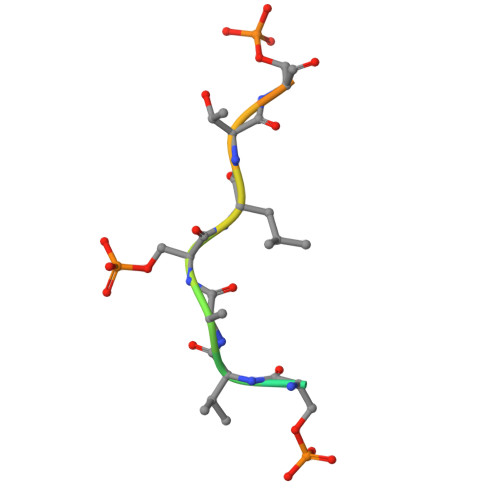> GKAESVASLTSQCSYA>KEPDPDKLKKAIVQVEHDERPARLILNRRPPAEGYAWLKYEDDGQEFEAN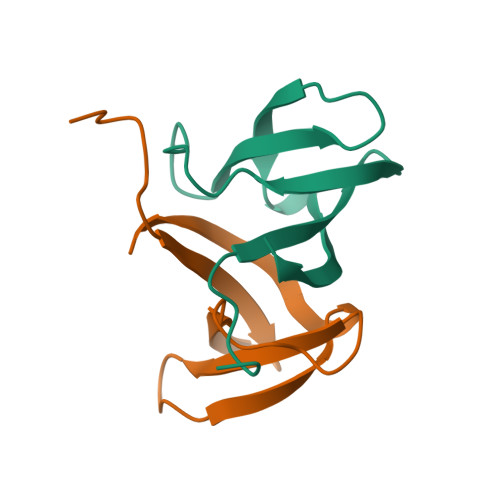LADVKLVALIEG[2x]>[4x]MALGTSGVKIHPNGNSNQLGVQLENVKLTSLFKKLDK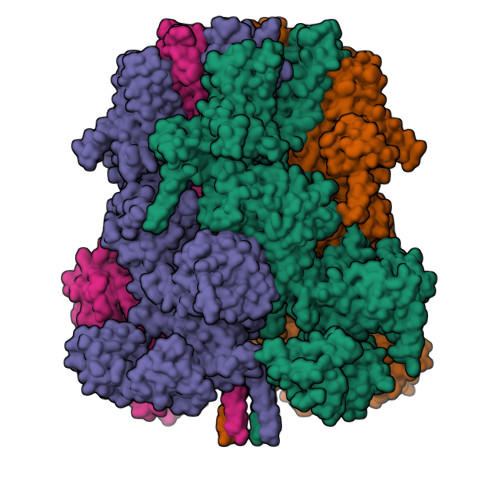RCSLASWIKENIKKKECCFYVEDGREGICKCGYPKVQHCDEAIKPEDYMGEQWDKHRHVRETPTDAFGDISFGGLGQKTGKYVRVSSDTSCENLYQLMTEQWKLRSPNLLISVTGGAKNFYIKTHLKDKFRRGLIKVAQTTGAWILTGGTHAGVMKHVGMAVRDYTLSSGSMEGQIVVIGVAPWGVIHNRSTLIHPEGRFPAYYSLDEQGQGRLSCLDINHTHFLLVDDGTQGHYGVEIELRARLEKLISKLSLGNRESGVTIPVVCVVLDGGPGTLNTIYNSMLNHTPCVVLEGSGRLADVIAHVASVPVSKVTMALINRLLKRFFMQEYKNFTELQIIEWTKKIQDILRMPHLLTVFRIDEDKNYDVDVAILQALLKASRSDEHAGRHCWERQLELAVAWNRVDIAESEIFTEESQWTSSDLHPAMFSALVGDKPEFVRLLLENGVCVREFLEREETLCELYSHLPSCFFLRKLAKRVQGGKMRRGQEPLPGSRKVCLSHVSEEVRHLLGSFTQPLYIASRYKPTKDDVRLKVPSKGALDLPCSGEEWSADTVWDPGRDLFLWAVVQNNRELAEIGWEQCRDCIAAALAASKILRKLAQESGEDDSEEATEMLELANHYEKQAIGVFSECHSWDAQRAQKLLIRISPSWGRSTCLWLALEAHDKSFIAHSGVQALLTQIWCGELSVDNPHWKVLLCMIFFPLIYTGFLTFRRDEDIQRQAERTEQQKLAMESVFAGQSDGKIKRHLRGFSQKSELKPLNCSSRLMSFLKSPQVKFYWNIASYFGFLWLFAVVLMIDFQTSPSWRELLLYVWLTSLVCEEIRQLYHDFDGSGFRRKAKMYIKDLWNILDVLSIVLFIAGLICRLQASDTVFYIGKVILCIDFIIFCLRLMAIFSISRTLGPKIIIVRRMMLDLFFFMFLLSIWVVAYGVAKQGILIENEERLNWIIRGAVYEPYITIFGNFPTNIDNTLFDISSCSVNASDPLKPKCPMLNADNTPVFPEWLTIMMLCVYLLFANILLLNLLIAIFNYTFQEVQDNTDTIWKFQRYELIKEYHSRPALPPPFILLSHLILFIRGVFLRDLPQRHKNFRQELEQTEEEELLSWEAYMKDNYLASTRQDESQSVEHRIHDTAEKVGAMSELLEREQEMVXXXXXXXXXXXXXXXXXXXXXXDEEAPHMFARQLQYPDSTVRRFPVPEEKVSWEVNFSPYQPPVYNQQDSSESDTSALDKHRNPGGRTGIRGKGALNTLGPNHILHPIFTRWRDAEHKVLEFLAVWEDAEKRWALLGGPAQPDEPLAQVLERILGKKLNEKTKTLLKAGEEVYKGYVDDSRNTDNAWVETSIITLHCDKNTPLMADLNHMVESSLSSHQPLQWREVSSDACRCSYQREALRQIAHHHNTYFSNSLEVLFQGPDYKDDDDKAHHHHHHHHHH> GDTETAIDNAIARVADTVASGPSNSTSIPALTAVETGHTSQVEPSDTMQTRHVKNYHSRSESTVENFLSRSACVYIEEYYTKDQDNVNRYMSWTINARRMVQLRRKFELFTYMRFDMEITFVITSRQLPGT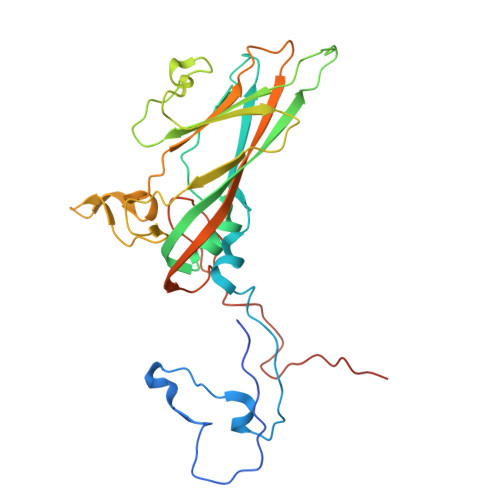SIAQDMPPLTHQIMYIPPGGPVPNSVTDFAWQTSTNPSIFWTEGNAPPRMSIPFISIGNAYSNFYDGWSHFSQNGVYGYNALNNMGKLYARHVNKDTPYQMSSTIRVYFKPKHIRVWVPRPPRLSPYIKSSNVNFNPTNLTDERSSITYVPDTIRPDVRTN>MGSSHHHHHHSSGLVPRGSHMPSYTVTVATGSQEHAGTDDYIYLSLVGSAGCSEKHLLDKGSFERGAVDSYDVTVDEELGEIQLVRIEKRKYGSNDDWYLKYITLKTPHGDYIEFPCYRWITGDVEVVLRDGRAKLARDDQIHILKQHRRKELETRQKQYRWMEWNPGFPLSIDAKCHKDLPRDIQFDSEKGVDFVLNYSKAMENLFINRFMHMFQSSWNDFADFEKIFVKISNTISERVMNHWQEDLMFGYQFLNGANPVLIRRCTELPEKLPVTTEMVECSLERQLSLEQEVQQGNIFIVDFELLDGIDANKTDPCTLQFLAAPICLLYKNLANKIVPIAIQLNQIPGDENPIFLPSDAKYDWLLAKIWVRSSDFHVHQTITHLLRTHLVSEVFGIAMYRQLPAVHPIFKLLVAHVRFTIAINTKAREQLICECGLFDKANATGGGGHVQMVQRAMKDLTYASLCFPEAIKARGMESKEDIPYYFYRDDGLLVWEAIRTFTAEVVDIYYEGDQVVEEDPELQDFVNDVYVYGMRGRKSSGFPKSVKSREQLSEYLTVVIFTASAQHAAVNFGQYDWASWIPNAPPTMRAPPPTAKGVVTIEQIVDTLPDRGRSCWHLGAVWALSQFQENELFLGMYPEEHFIEKPVKEAMARFRKNLEAIVSVIAERNENLQLPYYYLAPDRIPNSV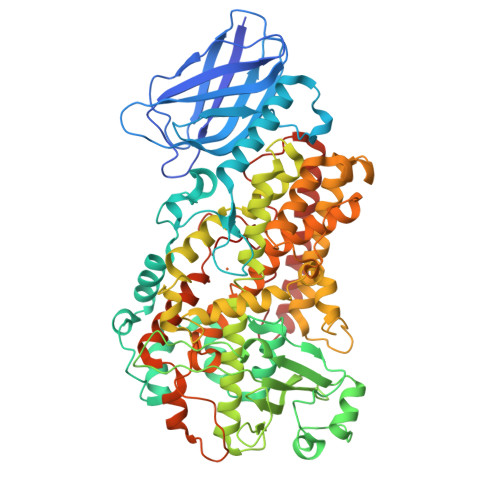AI[2x]>[2x]MAAPVVAPPGVVVSRANKRSGAGPGGSGGGGARGAEEEPPPPLQAVLVADSFDRRFFPISKDQPRVLLPLANVALIDYTLEFLTATGVQETFVFCCWKAAQIKEHLLKSKWCRPTSLNVVRIITSELYRSLGDVLRDVDAKALVRSDFLLVYGDVISNINITRALEEHRLRRKLEKNVSVMTMIFKESSPSHPTRCHEDNVVVAVDSTTNRVLHFQKTQGLRRFAFPLSLFQGSSDGVEVRYDLLDCHISICSPQVAQLFTDNFDYQTRDDFVRGLLVNEEILGNQIHMHVTAKEYGARVSNLHMYSAVCADVIRRWVYPLTPEANFTDSTTQSCTHSRHNIYRGPEVSLGHGSILEENVLLGSGTVIGSNCFITNSVIGPGCHIGDNVVLDQTYLWQGVRVAAGAQIHQSLLCDNAEVKERVTLKPRSVLTSQVVVGPNITLPEGSVISLHPPDAEEDEDDGEFSDDSGADQEKDKVKMKGYNPAEVGAAGKGYLWKAAGMNMEEEEELQQNLWGLKINMEEESESESEQSMDSEEPDSRGGSPQMDDIKVFQNEVLGTLQRGKEENISCDNLVLEINSLKYAYNISLKEVMQVLSHVVLEFPLQQMDSPLDSSRYCALLLPLLKAWSPVFRNYIKRAADHLEALAAIEDFFLEHEALGISMAKVLMAFYQLEILAEETILSWFSQRDTTDKGQQLRKNQQLQRFIQWLKEAEEESSEDD;>[2x]MPGSAAKGSELSERIESFVETLKRGGGPRSSEEMARETLGLLRQIITDHRWSNAGELMELIRREGRRMTAAQPSETTVGNMVRRVLKIIRE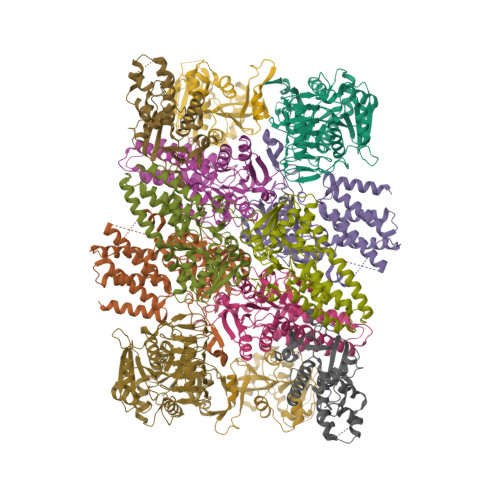EYGRLHGRSDESDQQESLHKLLTSGGLNEDFSFHYAQLQSNIIEAINELLVELEGTMENIAAQALEHIHSNEVIMTIGFSRTVEAFLKEAARKRKFHVIVAECAPFCQGHEMAVNLSKAGIETTVMTDAAIFAVMSRVNKVIIGTKTILANGALRAVTGTHTLALAAKHHSTPLIVCAPMFKLSPQFPNEEDSFHKFVAPEEVLPFTEGDILEKVSVHCPVFDYVPPELITLFISNIGGNAPSYIYRLMSELYHPDDHVL;>MAAVAVAVREDSGSGMKAELPPGPGAVGREMTKEEKLQLRKEKKQQKKKRKEEKGAEPETGSAVSAAQCQVGPTRELPESGIQLGTPREKVPAGRSKAELRAERRAKQEAERALKQARKGEQGGPPPKASPSTAGETPSGVKRLPEYPQVDDLLLRRLVKKPERQQVPTRKDYGSKVSLFSHLPQYSRQNSLTQFMSIPSSVIHPAMVRLGLQYSQGLVSGSNARCIALLRALQQVIQDYTTPPNEELSRDLVNKLKPYMSFLTQCRPLSASMHNAIKFLNKEITSVGSSKREEEAKSELRAAIDRYVQEKIVLAAQAISRFAYQKISNGDVILVYGCSSLVSRILQEAWTEGRRFRVVVVDSRPWLEGRHTLRSLVHAGVPASYLLIPAASYVLPEVSKVLLGAHALLANGSVMSRVGTAQLALVARAHNVPVLVCCETYKFCERVQTDAFVSNELDDPDDLQCKRGEHVALANWQNHASLRLLNLVYDVTPPELVDLVITELGMIPCSSVPVVLRVKSSDQ[2x];>[2x]MDDKELIEYFKSQMKEDPDMASAVAAIRTLLEFLKRDKGETIQGLRANLTSAIETLCGVDSSVAVSSGGELFLRFISLASLEYSDYSKCKKIMIERGELFLRRISLSRNKIADLCHTFIKDGATILTHAYSRVVLRVLEAAVAAKKRFSVYVTESQPDLSGKKMAKALCHLNVPVTVVLDAAVGYIMEKADLVIVGAEGVVENGGIINKIGTNQMAVCAKAQNKPFYVVAESFKFVRLFPLNQQDVPDKFKYKADTLKVAQTGQDLKEEHPWVDYTAPSLITLLFTDLGVLTPSAVSDELIKLYL;>MEFQAVVMAVGGGSRMTDLTSSIPKPLLPVGNKPLIWYPLNLLERVGFEEVIVVTTRDVQKALCAEFKMKMKPDIVCIPDDADMGTADSLRYIYPKLKTDVLVLSCDLITDVALHEVVDLFRAYDASLAMLMRKGQDSIEPVPGQKGKKKAVEQRDFIGVDSTGKRLLFMANEADLDEELVIKGSILQKHPRIRFHTGLVDAHLYCLKKYIVDFLMENGSITSIRSELIPYLVRKQFSSASSQQGQEEKEEDLKKKELKSLDIYSFIKEANTLNLAPYDACWNACRGDRWEDLSRSQVRCYVHIMKEGLCSRVSTLGLYMEANRQVPKLLSALCPEEPPVHSSAQIVSKHLVGVDSLIGPETQIGEKSSIKRSVIGSSCLIKDRVTITNCLLMNSVTVEEGSNIQGSVICNNAVIEKGADIKDCLIGSGQRIEAKAKRVNEVIVGNDQLMEI[2x];>MNSQYMFDYPAINIDVRCHRLLSSVSYVAYNKFHTHDVSTYEHCEIPLEKLRLGFGRRNSLADFYSLGELPASWGPACYFSSVKPMMYTFQGMASDLSRFDLTSFSRKGLPNVLKALSWPLGIPDCEIFSICSDRFVRGLQTRDQLMSYILRMGDSHSLDECIVQAHKKILQEARRLGLSDEHYNGYDLFREIGSLVCLRLINAEPFDTASSGEALDVRTVIRSYRASDPSTGLTEYGNSLWTPIHSHVDENDESSSDSDFGSHHHHHH[2x]>PPGPPGPPGPPGPPGPPGPPG[6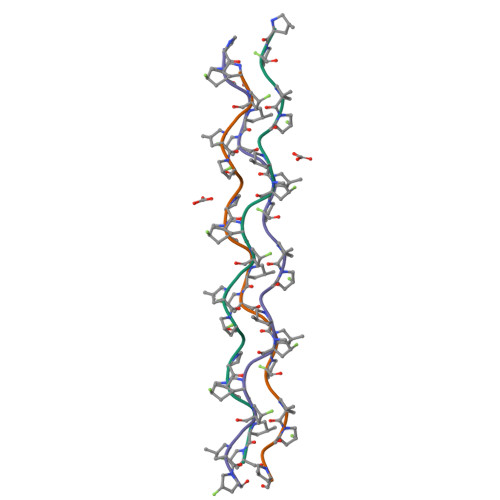x]>SLGGARRFLCGVVEGFYGRPWVMEQRKELFRRLQKWELNTYLYAPKDDYKHRMFWREMYSVEEAEQLMTLISAAREYEIEFIYAISPGLDITFSNPKEVSTLKRKLDQVSQFGCRSFALLFDDIDHNMCAADKEVFSSFAHAQVSITNEIYQYLGEPETFLFCPTEYCGTFCYPNVSQSPYLRTVGEKLLPGIEVLWTGPKVVSKEIPVESIEEVSKIIKRAPVIWDNIHANDYDQKRLFLGPYKGRSTELIPRLKGVLTNPNCEFEANYVAIHTLATWYKSNMNYSPQMALKLALTEWLQEFGVPHQYSSRQVAHSGAKASVVDPGPNEKPLYT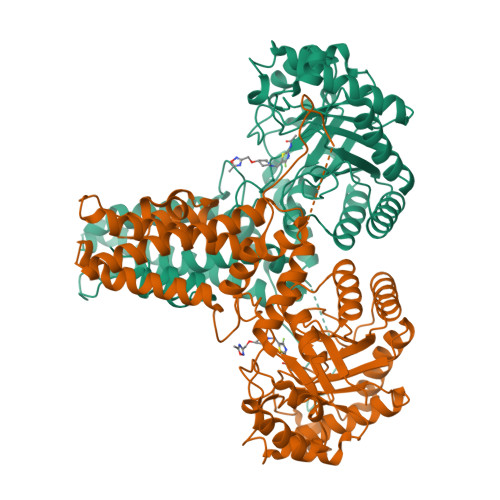AEPVTLEDLQLLADLFYLPYEHGPKGAQMLREFQWLRANSSVVSVNSKGKDSEKIEEWRSRAAKFEEMCGLVMGMFTRLSNCANRTILYDMYSYVWDIKSIMSMVKSFVQWLGERSHSSAQFLIGDQEPWAFRGGLAGEFQRLLPIDGANDLFFQPPPLTPTSK[2x]>[2x]SHMKYLIGANFKMYKSHKDLQEYFDQFVNNYACFVNIDLMIAPMTVCLGTASEMTKDSCVHLGAQNMHYEDQGAYTGETSPLILKELGAEYVI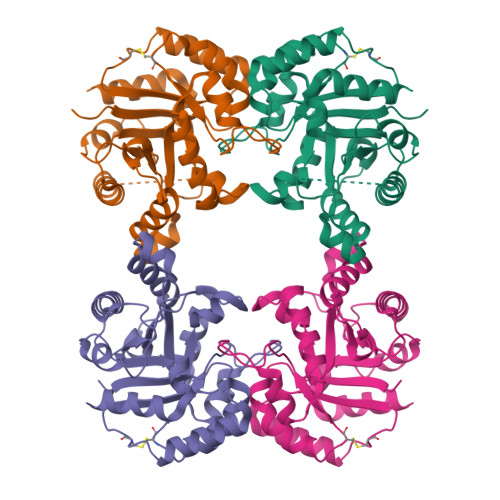IGHSERRQYFGETNQMINKKLKSALQHGIRPILCIGENLEQKELGISKETLKIQLREALQGIDTLDQIDVAYEPVRAIGTGKSATPEEVQDIHEYIRSVLGNEKSRIIYGGSVNDTNADILIAQPAVNGFLIGSASLDPQKFLKILDVVSKKNK> GMKQDSIITLHPDDRSEQTAEIMRRFNDVFQLHDPAALPELIAEECVIENTVPAPDGARHAGRQACV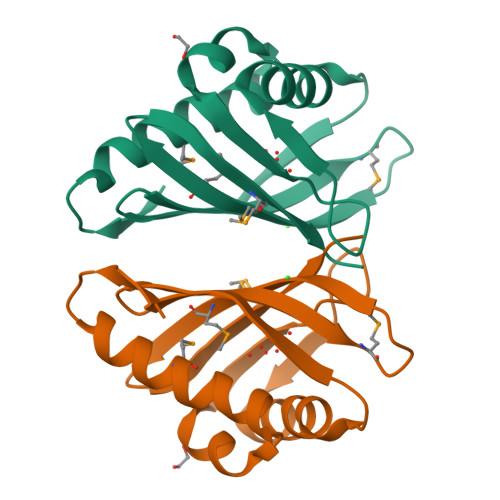QLWSAIATQPGTRFDLEETFVAGDRATIRWRYWMADGNSVRGVNLMRVQDGRIVEAMGYVKG> AWTQEKNHHQPAHLNSSSLQQVA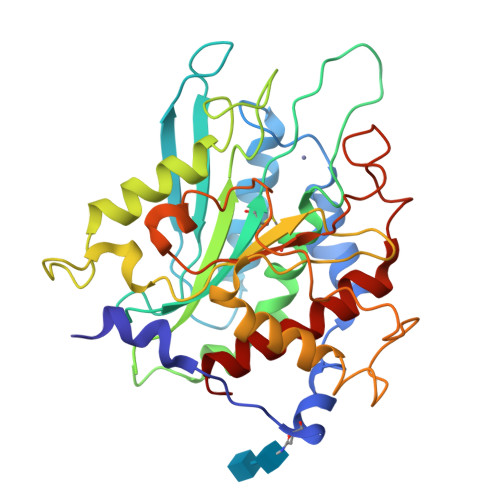EGTSISEMWQNDLRPLLIERYPGSPGSYSARQHIMQRIQRLQAEWVVEVDTFLSRTPYGYRSFSNIISTLNPEAKRHLVLACHYDSKYFPRWDSRVFVGATDSAVPCAMMLELARALDKKLHSLKDVSGSKPDLSLRLIFFDGEEAFHHWSPQDSLYGSRHLAQKMASSPHPPGSRGTNQLDGMDLLVLLDLIGAANPTFPNFFPKTTRWFNRLQAIEKELYELGLLKDHSLERKYFQNFGYGNIIQDDHIPFLRKGVPVLHLIASPFPEVWHTMDDNEENLHASTIDNLNKIIQVFVLEYLHL>[2x]NASGERLSQLLKKLFETQESGDLNEELVKAAANGDVAKVEDLLKRPDVDVNGQCAGHTAMQAASQNGHVDILKLLLKQNVDVEAEDKDGDRAVHHAAFGDEGAVIEVLHRGSADLNARNKRRQTPLHIAVNKGHLQVVKTLLDFGCHPSLQDSEGDTPLHDAISKKRDDILAVLLEAGADVTITNNNGFNALHHAALRGNP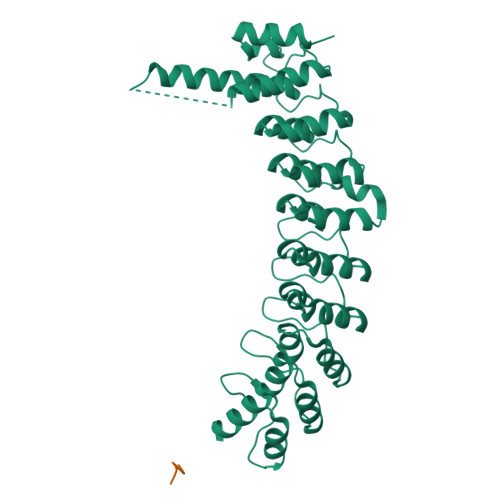SAMRVLLSKLPRPWIVDEKKDDGYTALHLAALNNHVEVAELLVHQGNANLDIQNVNQQTALHLAVERQHTQIVRLLVRAGAKLDIQDKDGDTPLHEALRHHTLSQLRQLQDMQDVGKVDAAWEPSKNTLIMGLGTQGAEKKSAASIACFLAANGADLSIRNKKGQSPLDLCPDPNLCKALAKCHK> SINGGIRAATSQEINELTYYTTLSANSYCRTVIPGATWDCIHCDATEDLKIIKTWSTLIYDTNAMVARGDSEKTIYIVFRGSSSIRNWIADLTFVPVSYPPVSGTKVHKGFLDSYGEVQNELVATVLDQFKQYPSYKVAVTGHSLGGATVLLCALDLYQREEGLSSSNLFLYTQGQPRVGDPAFANYVVSTGIPYRRTVNERDIVPHLPPAAFGFLHAGEEYWITDNSPETVQVC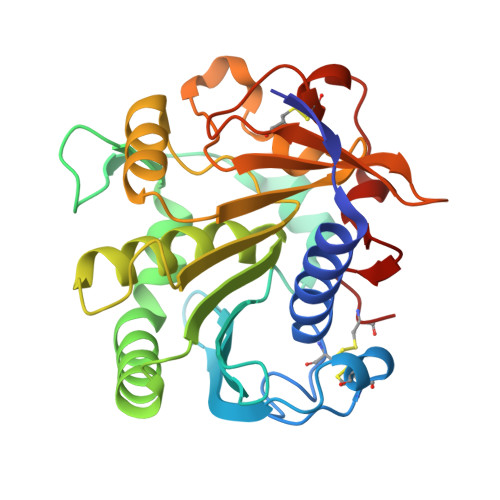TSDLETSDCSNSIVPFTSVLDHLSYFGINTGLCT3-oxo-3-[(3R)-3-(pyrrolo[2,3-b][1,2,3]triazolo[4,5-d]pyridin-1(6H)-yl)piperidin-1-yl]propanenitrile 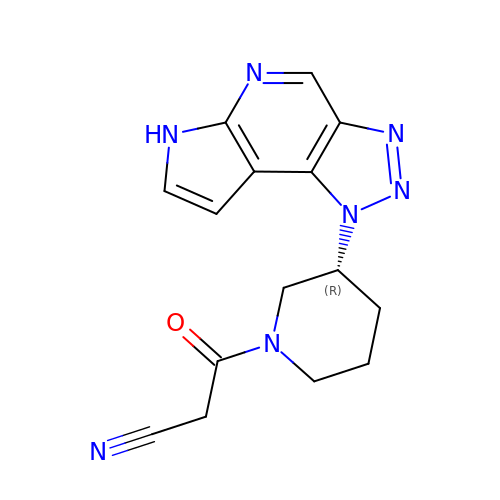| C15 H15 N7 O | COGIAVJREKAVDL-SNVBAGLBSA-N> MVPISPIETVPVKLKPGMDGPKVKQWPLTEEKIKALVEICTEMEKEGKISKIGPENPYNTPVFAIKKKDSTKWRKLVDFRELNKRTQDFWEVQLGIPHPAGLKKKKSVTVLDVGDAYFSVPLDEDFRKYTAFTIPSINNETPGIRYQYNVLPQGWKGSPAIFQSSMTKILEPFAAQNPDIVIYQYMDDLYVGSDLEIGQHRTKIEELRQHLLRWGLTTPDKKHQKEPPFLWMGYELHPDKWTVQPIVLPEKDSWTVNDIQKLVGKLNWASQIYPGIKVRQLSKLLRGTKALTEVIPLTEEAELELAENREILKEPVHGVYYDPSKDLIAEIQKQGQGQWTYQIYQEPFKNLKTGKYARMRGAHTNDVKQLTEAVQKITTESIVIWGKTPKFKLPIQKETWETWWTEYWQATWIPEWEFVNTPPLVKLWYQLEKEPIVGAETFYVDGAANRETKLGKAGYVTNKGRQKVVPLTNTTNQKTELQAIYLALQDSGLEVNIVTDSQYALGIIQAQPDKSESELVNQIIEQLIKKEKVYLAWVPAHKGIGGNEQVDKLVSAG;> PISPIETVPVKLKPGMDGPKVKQWPLTEEKIKALVEICTEMEKEGKISKIGPENPYNTPVFAIKKKDSTKWRKLVDFRELNKRTQD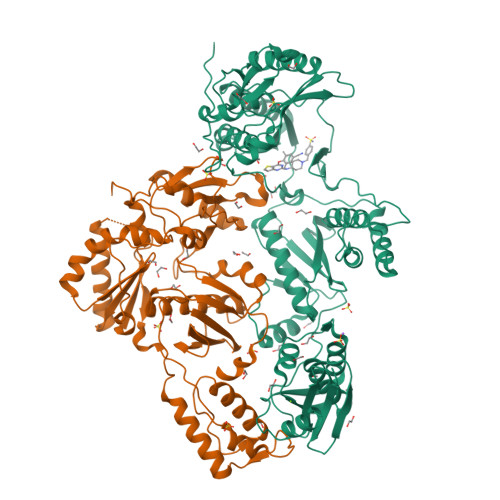FWEVQLGIPHPAGLKKKKSVTVLDVGDAYFSVPLDEDFRKYTAFTIPSINNKTPGIRYQYNVLPQGWKGSPAIFQSSMTKILEPFKKQNPDIVIYQYMDDLYVGSDLEIGQHRTKIEELRQHLLRWGLTTPDKKHQKEPPFLWMGYELHPDKWTVQPIVLPEKDSWTVNDIQKLVGKLNWASQIYPGIKVRQLSKLLRGTKALTEVIPLTEEAELELAENREILKEPVHGVYYDPSKDLIAEIQKQGQGQWTYQIYQEPFKNLKTGKYARMRGAHTNDVKQLTEAVQKITTESIVIWGKTPKFKLPIQKETWETWWTEYWQATWIPEWEFVNTPPLVKLWYQ2-(3,4-dihydroxyphenyl)-5,7-dihydroxy-4-oxo-4H-chromen-3-yl 6-deoxy-alpha-L-mannopyranoside | C21 H20 O11 | 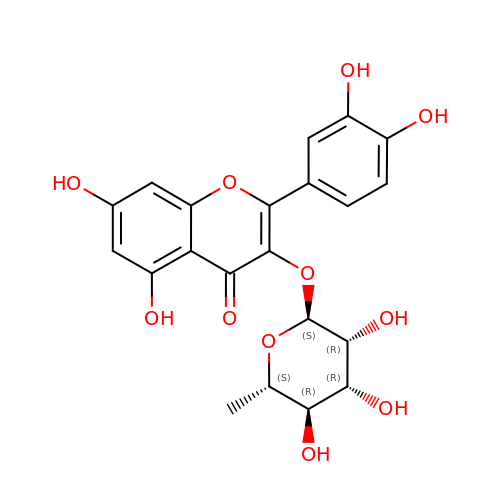OXGUCUVFOIWWQJ-HQBVPOQASA-N> TVAYIAIGSNLASPLEQVNAALKALGDIPESHILTVSSFYRTPPLGPQDQPDYLNAAVALETSLAPEELLNHTQRIELQQGRVR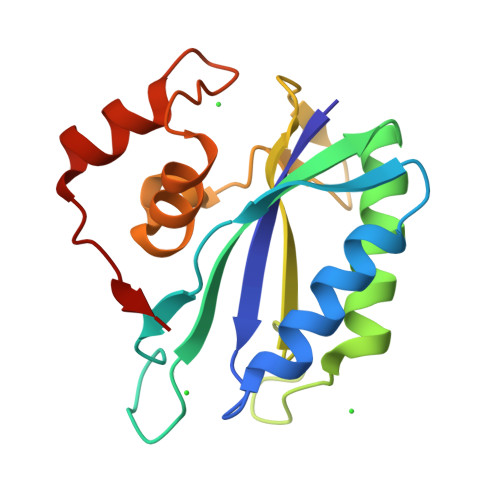KAERWGPRTLDLAIMLFGNEVINTERLTVPHYDMKNRGFMLWPLFEIAPELVFPDGEMLRQILHTRAFDKLNKW>HMRVL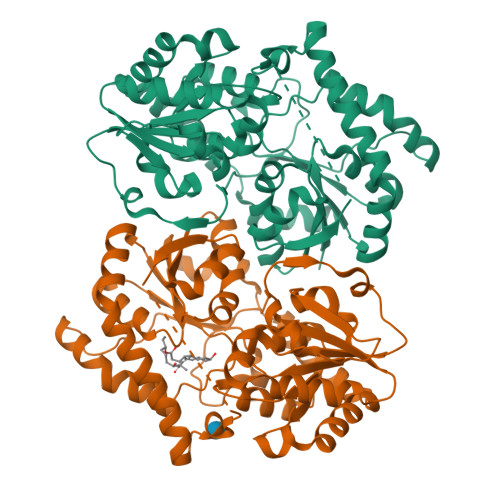VVPLPYPTHLMAMVPLCWALQASGHEVLIAAPPELQATAHGAGLTTAGIRGNDRTGDTGGTTQLRFPNPAFGQRDTEAGRQLWEQTASNVAQSSLDQLPEYLRLAEAWRPSVLLVDVCALIGRVLGGLLDLPVVLHRWGVDPTAGPFSDRAHELLDPVCRHHGLTGLPTPELILDPCPPSLQASDAPQGAPVQYVPYNGSGAFPAWGAARTSARRVCICMGRMVLNATGPAPLLRAVAAATELPGVEAVIAVPPEHRALLTDLPDNARIAESVPLNLFLRTCELVICAGGSGTAFTATRLGIPQLVLPQYFDQFDYARNLAAAGAGICLPDEQAQSDHEQFTDSIATVLGDTGFAAAAIKLSDEITAMPHPAALVRTLENTA[2x]>MKTPEDCTGLADIREAIDRIDLDIVQALGRRMDYVKAASRFKASEAAIPAPERVAAMLPERARWAEENGLDAPFVEGLFAQIIHWYIAEQIKYW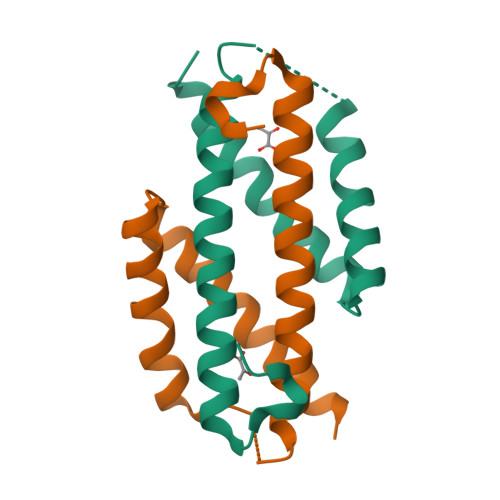RQTRGAA[4x]>MPMCGGLTTSVRPSNEDKQLLTPVVKDYIAQQLGREPSEVKITEVSRQIVNGTNHFLKVEHDGNCWHVRVHE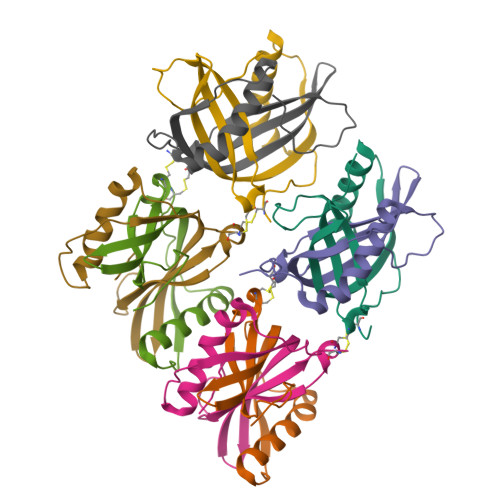ALPCYGGKVEVHSHKVASVGDPLTYFLEHHHHHH[8x]>GATESGKRMDCPALP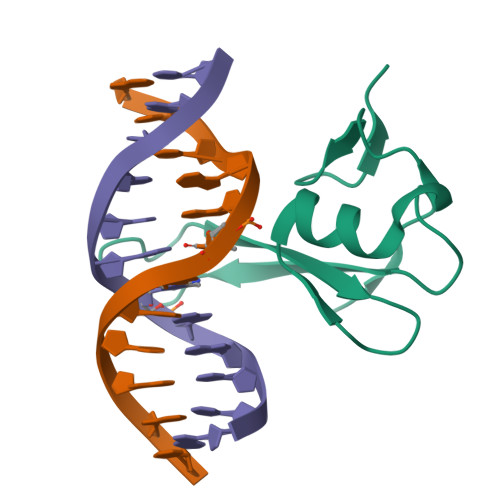PGWKKEEVIRKSGLSAGKSDVYYFSPSGKKFRSKPQLARYLGNTVDLSSFDFRTGKMMPSKLQK[2x]> ADTVTLPFANGERPLVMYPGKRPLIGLTARPPQLETPFSVFDEGLITPNDAFFVMYHLAGIPLEIDPDAFRLEIKGKVGTPLSLSLQDLKNDFPASEVVAVNQCSGNSRGFVEPRVGGGQLANGAMGNARWRGVPLKAVLEKAGVQAGAKQ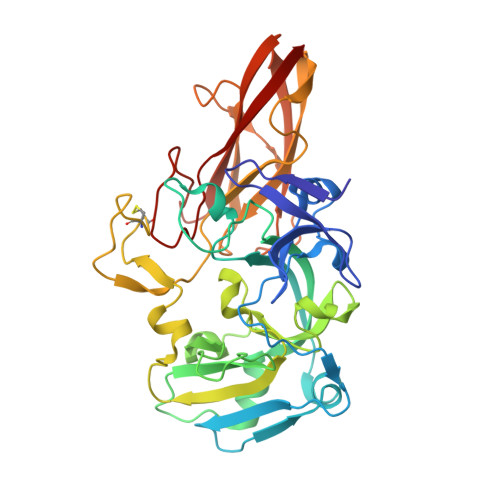VTFGGLDGPVIPETPDFVKALSIDHATDGEVMLAYSMNGADLPWLNGYPLRLVVPGYYGTYWVKHLNEITVIDKEFDGFWMKTAYRIPDNACACTEPGKAPTATIPINRFDVRSFITNVENGASVKAGEVPLRGIAFDGGYGITQVSVSADAGKSWTNATLDPGLGKYSFRGWKAVLPLTKGDHVLMCRATNARGETQPMQATWNPAGYMRNVVEATRVIAA> MNHKVHHHHHHHHMATFISVQLKKTSEVDLAKPLVKFIQQTYPSGGEEQAQYCRAAEELSKLRRAAVGRPLDKHEGALETLLRYYDQICSIEPKFPFSENQICLTFTWKDAFDKGSLFGGSVKLALASLGYEKSCVLFNCAALASQIAAEQNLDNDEGLKIAAKHYQFASGAFLHIKETVLSALSREPTVDISPDTVGTLSLIMLAQAQEVFFLKATRDKMKDAIIAKLANQAADYFGDAFKQCQYKDTLPKEVFPVLAAKHCIMQANAEYHQSILAKQQKKFGEEIARLQHAAELIKTVASRYDEYVNVKDFSDKINRALAAAKKDNDFIYHDRVPDLKDLDPIGKATLVKSTPVNVPISQKFTDLFEKMV;> MNHKVHHHHHHHHMLETLINKIYTGPLGEELVQTLYLRIWAMEETPESLKILQMREDIRDQVLKMKTERWLRTLIRGEKTKLKDFQKRYEEVHPYLMKEKVEQVIMEEAWS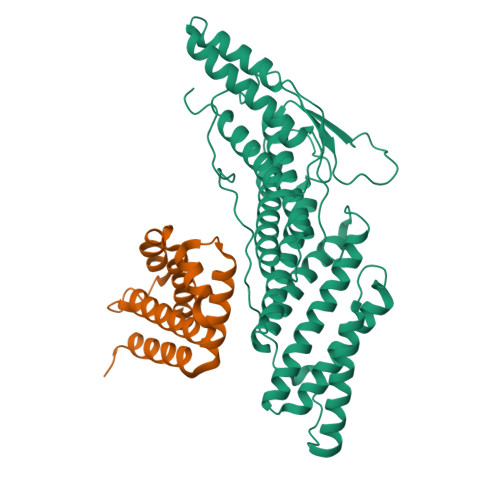LAAHIVQE>GSSPEKPTPNGGIPHDNLVLIRMKPDENGRFGFNVKGGYDQKMPVIVSRVAPGTPADLCVPRLNEG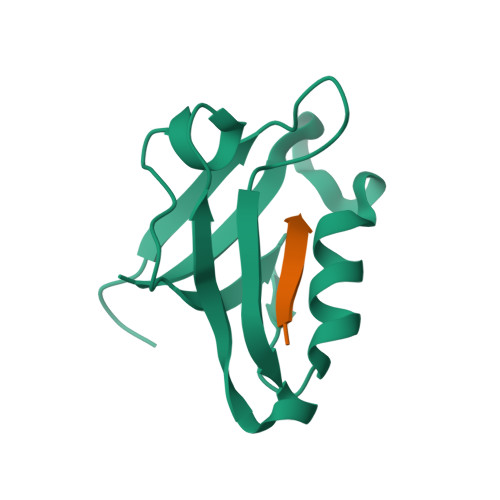DQVVLINGRDIAEHTHDQVVLFIKASCERHSGELMLLVRPN[4x];>SNRRVYKKMPSIESDV[4x]>[13x]MISQSRYIRIISGVGAGAPVAGRKLILRVMTTNNVIPPGIVIEFDNANAVLSYFGAQSEEYQRAAAYFKFISKSVNSPSSISFARWVNTAIAPMVVGDNLPKTIADFAGFSAGVLTIMVGAAEQNITAIDTSAATSMDNVASIIQTEIRKNADPQLAQATVTWNQN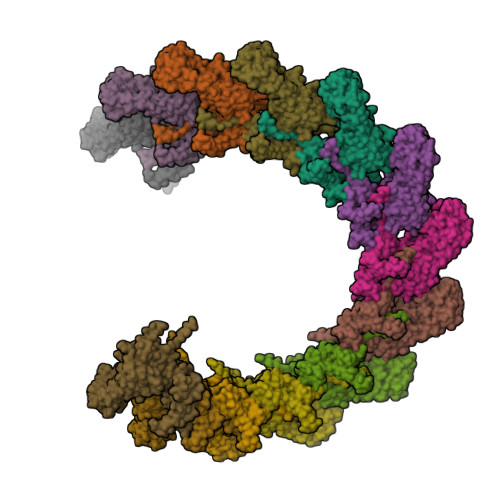TNQFTLVGATIGTGVLAVAKSADPQDMSTALGWSTSNVVNVAGQSADLPDAAVAKSTNVSNNFGSFLFAGAPLDNDQIKAVSAWNAAQNNQFIYTVATSLANLGTLFTLVNGNAGTALNVLSATAANDFVEQCPSEILAATNYDEPGASQNYMYYQFPGRNITVSDDTVANTVDKSRGNYIGVTQANGQQLAFYQRGILCGGPTDAVDMNVYANEIWLKSAIAQALLDLFLNVNAVPASSTGEAMTLAVLQPVLDKATANGTFTYGKEISAVQQQYITQVTGDRRAWRQVQTLGYWINITFSSYTNSNTGLTEWKANYTLIYSKGDAIRFVEGSDVMI> MGNFIITERKKAKEERSNPQTDSMDDLLIRRLTDRNDKEA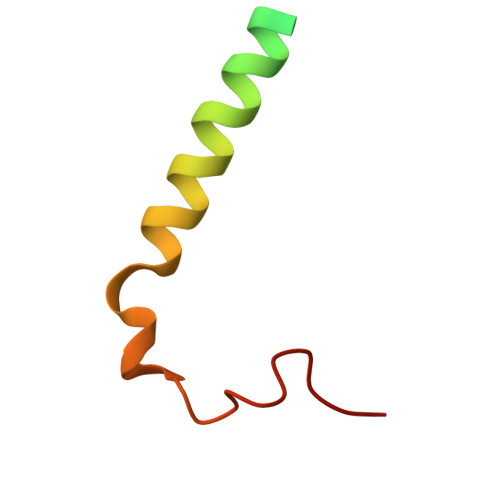HLNELFQDNSGAIGGNI> YQEPTDPKFPQQWYLSGVTQRDLNVKAAWAQGYTGHGIVVSILDDGIEKNHPDLAGNYDPGASFDVNDQDPDPQPRYTQMNDNRHGTRCAGEVAAVANNGVCGVGVAYNARIGGVRMLDGEVTDAVEARSLGLNPNHIHIYSASWGPEDDGKTVDGPARLAEEAFFRGVSQGRGGLGSIFVWASGNGGREHDSCNCDGYTNSIYTLSISSATQFGNVPWYSEACSSTLATTYSSGNQNEKQIVTTDLRQKCTESHTGTSASAPLAAGIIALTLEANKDLTWRDMQHLVVQTSKPAHLNANDWATNGVGRKVSHSYGYGLLDAGAMVALAQDWTTVAPQRKCIIDILTE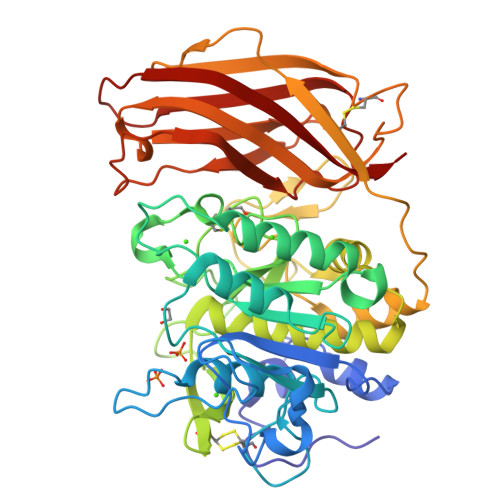PKDIGKRLEVRKTVTACLGEPNHITRLEHAQARLTLSYNRRGDLAIHLVSPMGTRSTLLAARPHDYSADGFNDWAFMTTHSWDEDPSGEWVLEIENTSEANNYGTLTKFTLVLYGTA>MIEERLEALQSESHRLENALSIIEEERKQLKLKEAELQEEYQNSLRPLQQLQYLTLSACEEEKRQELMYEIGQIGDLIEDWATDKREALKREEGRIEDKQNELFYKRQKLILEVEEQKKDKESTDG[4x]

Bacterial type VIIb secretion systems (T7SSb) are multisubunit integral membrane protein complexes found in Firmicutes that play a role in both bacterial competition and virulence by secreting toxic effector proteins. The majority of characterized T7SSb effectors adopt a polymorphic domain architecture consisting of a conserved N-terminal Leu-X-Gly (LXG) domain and a variable C-terminal toxin domain. Using coimmunoprecipitation-mass spectrometry analyses, in vitro copurification experiments, and T7SSb secretion assays, we found that representative members of these protein families form heteromeric complexes with their cognate LXG domain and in doing so, function as targeting factors that promote effector export. Additionally, an X-ray crystal structure of a representative DUF3958 protein, combined with predictive modeling of DUF3130 using AlphaFold2, revealed structural similarity between these protein families and the ubiquitous WXG100 family of T7SS effectors.

Despite this discouraging trend, LapD2 was the sole exception and after systematic optimization of its crystallization conditions it formed crystals that diffracted to 2.2 Å. The crystallographic phase problem was overcome using selenomethionine-incorporated protein and the single wavelength anomalous dispersion (SAD) technique. The overall structure of LapD2 shows that it adopts a helix-turn-helix fold that is reminiscent of the WXG100 family of small secreted T7SS effectors. However, in contrast to characterized WXG100 proteins, which typically form head-to-toe homodimers mediated by hydrophobic interactions, the turn region of LapD2 contains an intermolecular disulfide bond formed by cysteine 59 that facilitates head-to-head dimerization. The head region of LapD2 also possesses a hydrophobic patch that may contribute to dimerization. Not surprisingly, the energy of head-to-head dimer formation as predicted by the PDBePISA webtool is highly favorable (ΔiG = −21.0) due to the combined effects of burying a hydrophobic patch from the aqueous milieu and possessing a disulfide linkage. PDBePISA also revealed a toe-to-toe homodimer interface, and this interaction was also suggested to be favorable, although with a lower energy of formation (ΔiG = −11.6). Notably, conservation is very low within the interhelical turn region, which contrasts with the highly conserved WXG motif found within structurally similar WXG100 proteins. One of the more striking features of LapD2 is the disulfide bond formed by Cys59 that contributes to dimerization. This residue is not conserved among Lap2 proteins indicating that an intermolecular disulfide bond is likely not a universal property of this protein family. Consistent with not playing an important role in LapD2 function, we found that an S. intermedius GC1825 ΔlapD2 strain expressing plasmid-borne LapD2C59S secretes wild-type levels of TelD.> MKTQVAIIGAGPSGLLLGQLLHKAGIDNVILERQTPDYVLGRIKAGVLEQGMVDLLREAGVDRRMARDGLVHEGVEIAFAGQRRRIDLKRLSGGKTVTVYGQTEVTRDLMEAREASGATTVYQAAEVRLHDLQGERPYVTFERDGERLRLDCDYIAGCDGFHGISRQSIPAERLKVFERVYPFGWLGLLADTPPVSHELIYANHPRGFALCSQRSATRSRYYVQVPLTEKVEDWSDERFWTELKARLPAEVAEKLVTGPSLEKSIAPLRSFVVEPMQHGRLFLAGDAAHIVPPTGAKGLNLAASDVSTLYRLLLKAYREGRGEL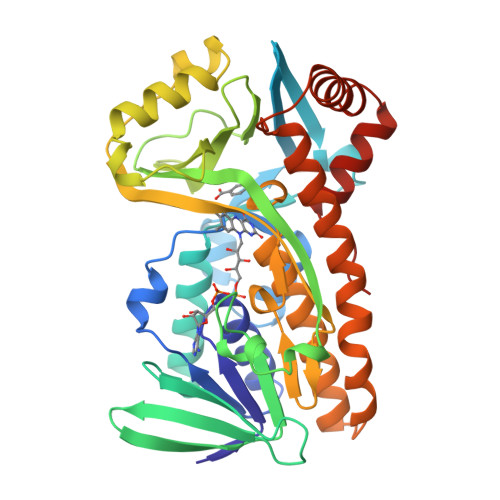LERYSAICLRRIWKAERFSWWMTSVLHRFPDTDAFSQRIQQTELEYYLGSEAGLATIAENYVGLPYEEIE>[4x]MKRKIIFLASPYGFSQQQKTLLLPPIVRALEALGIEVWEPFARNNQIDFSQADWAYRVAQADLQDVKNCDGIFAVVNGTPPDEGVMVELGMAIALNKAIFLFRDDFRRCSDNERYPLNLMLFAGLPEIGWENYYYTSVDEIQSHDKALYKWLTG

Guided by the structure of the enzyme from the thermophilic organism Chroococcidiopsis thermalis PCC 7203 (CtNDT) bound to the ribonucleoside analogue Immucillin-H, we designed mutants of CtNDT and the psychrotolerant Bacillus psychrosaccharolyticus (BpNDT) to improve catalytic efficiency with 3′-deoxynucleosides and ribonucleosides, while maintaining nucleobase promiscuity to generate over 100 distinct nucleoside products. CtNDT has a preference for purine-based 2′-deoxynucleosides, while BpNDT prefers pyrimidine-based 2′-deoxynucleosides. Importantly, wild type CtNDT can utilize ribonucleoside and 3′-deoxynucleoside substrates, albeit with lower efficiency, demonstrating less strict selection of 2′-deoxynucleosides, and a possible strategy to produce 3′-deoxynucleosides. , As proof of concept, we determined cordycepin (3′-deoxyadenosine), a natural product currently employed to treat various types of cancers, can be used as a substrate by CtNDT. We have previously shown that this tyrosine residue in CtNDT (Y7) does not directly interact with the 2′-OH group, and instead positions the catalytic E88 for reaction.

To understand the interaction between CtNDT and ribonucleosides, we cocrystallized the variant CtNDTY7F, which possesses higher catalytic efficiency with ribonucleoside substrates than CtNDTWT with the nucleoside analogue Immucillin-H (ImmH). This analogue is a purine nucleoside phosphorylase inhibitor, rationally designed to mimic the transition state of the reaction catalyzed by that enzyme. Importantly, for CtNDT it is a nonhydrolyzable substrate analogue containing hydroxyl groups on positions 2′ and 3′. Figure a compares the structures of CtNDTWT and CtNDTY7F, depicting key residues participating in the reaction and substrate selection. A flexible loop that acts as a “lid” and could potentially allow bulkier substrates to be used was observed in an “open” or “closed” conformation. Figure S3e depicts differences in the normalized B-factors for this flexible loop and ligands, as only 2 molecules of ImmH were placed in the CtNDTY7F tetramer, with less defined electron density in the nucleobase moiety of ImmH, while two other monomers remained unoccupied. No major differences are present in the protein backbone, but the wild-type enzyme binds ImmH in a distorted conformation in relation to the ribose ring, bringing the 2′-OH farther from D62 and closer to Y7, likely to avoid clashes, which does not occur in the CtNDTY7F mutant. Following our interaction map with ImmH, a ribonucleoside analogue, we designed mutants targeting residues surrounding the 2′-OH group, aimed at further tailoring substrate selection toward modified sugars.>[6x]MGSSHHHHHHSQDPNSRHYTSLTFGPINPSIPSSYAPSGISHLLSRQLVVVYGPDAAKYLQGMVTANVYMPGSGSM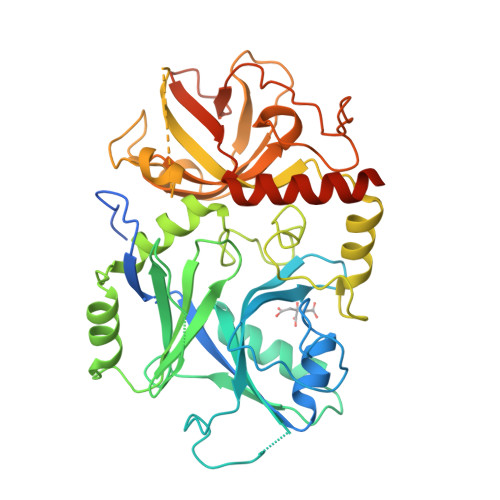VRTDRGYYAALLTGQGRVLYDVFIYPLTDSKHLQRVLPSADVEGAAFLIEVDKDQAGLLVDHIKRYRVRAKVKVKVVDVEEVAVWHAWDPNGLGEASVNDLLVTPDCRTPAMGSRILHFGGPDGNAIQNFAERCQLQVLPQEYYVLHRITQGVPEGQTELLKMSAIPHESNLDLMGGIDFRKGCYVGQELVTRTEHRGVVRKRVLPCVVYEGSQGQAVDIRATGGDLGGLYTDRPIAGLSSAREIASETNIVRVSGKGRGVGKWLRGIGNVGLAVCRLDVMTDLPIPGETPAGEDGVPEVREVKGEFTIEGDEGPLRIKAVPPAWLRRELMEKWEVKNEQNMVRFQREAIESEEEM>MAEELVLERCDLELETNGRDHHTADLCREKLVVRRGQPFWLTLHFEGRNYEASVDSLTFSVVTGPAPSQEAGTKARFPLRDAVEEGDWTATVVDQQDCTLSLQLTTPANAPIGLYRLSLEASTGYQGSSFVLGHFILLFNAWCPADAVYLDSEEERQEYVLTQQGFIYQGSAKFIKNIPWNFGQFEDGILDICLILLDVNPKFLKNAGRDCSRRSSPVYVGRVVSGMVNCNDDQGVLLGRWDNNYGDGVSPMSWIGSVDILRRWKNHGCQRVKYGQCWVFAAVACTVLRCLGIPTRVVTNYNSAHDQNSNLLIEYFRNEFGEIQGDKSEMIWNFHCWVESWMTRPDLQPGYEGWQALDPTPQEKSEGTYCCGPVPVRAIKEGDLSTKYDAPFVFAEVNADVVDWIQQDDGSVHKSINRSLIVGLKISTKSVGRDEREDITHTYKYPEGSSEEREAFTRANHLNKLAEKEETGMAMRIRVGQSMNMGSDFDVFAHITNNTAEEYVCRLLLCARTVSYNGILGPECGTKYLLNLNLEPFSEKSVPLCILYEKYRDCLTESNLIKVRALLVEPVINSYLLAERDLYLENPEIKIRILGEPKQKRKLVAEVSLQNPLPVALEGCTFTVEGAGLTEEQKTVEIPDPVEAGEEVKVRMDLLPLHMGLHKLVVNFESDKLKAVKGFRNVIIGPA[3x]

Transglutaminase 2 (TG2) is a calcium-dependent enzyme that regulates many biological processes, including apoptosis, autophagy, inflammation, and extracellular matrix formation. TG2 is regulated by the binding of guanine nucleotides and Ca2+. The transamidation activity of TG2 is inhibited by GTP or GDP binding, which stabilizes its closed structure, thereby obstructing the accessibility of substrates to the active sites. In contrast, Ca2+ acts as a cofactor in the transamidation activity by inducing conformational change to the active open form.

To identify the Ca2+ binding sites, a Ca2+-containing crystal of TG2 was produced in totally different crystallization conditions from those used for the previous structural study of TG2. A relatively low-resolution structure of 3.56 Å was solved and refined to Rwork = 22.5% and Rfree = 26.3%. The structure revealed that the asymmetric unit (ASU) cell contained three molecules. The final structural models were constructed with residues 2-687 for chain A, residues 3-687 for chain B, and residues 9-687 for chain C. GDP was detected at the nucleotide binding site in each chain. After careful analysis by comparing the current structure with previous TG2 structures that do not contain Ca2+, we identified two tentative Ca2+ binding sites in the structure of TG2. The first binding site is located in the catalytic domain and is coordinated by the side chains of E437, Y159, and E155. The second binding site is located in the β-barrel 1 domain and is coordinated by the main chains of N497 and F537, and side chains of E539 and N498. Binding of Ca2+ to E437 and E539 induced some structural changes in two loops of TG2, amino acids 406–412 and 460–470. Thus, binding of Ca2+ to E437 and E539 is likely to promote an open active conformation of TG2 by altering the hinge structure. Intriguingly, the present Ca2+ bound TG2 crystal structure is a GDP-bound compact form that binds Ca2+ at only two sites, namely, E437 and E539.1-(4-methoxybutyl)-~{N}-(2-methylpropyl)-~{N}-[(3~{S},5~{R})-5-morpholin-4-ylcarbonylpiperidin-3-yl]benzimidazole-2-carboxamide | C27 H41 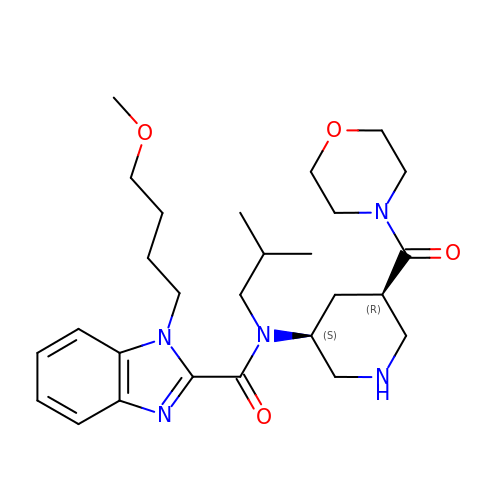N5 O4 | RHIBAIKQWJNESW-YADHBBJMSA-N> WKEPCRI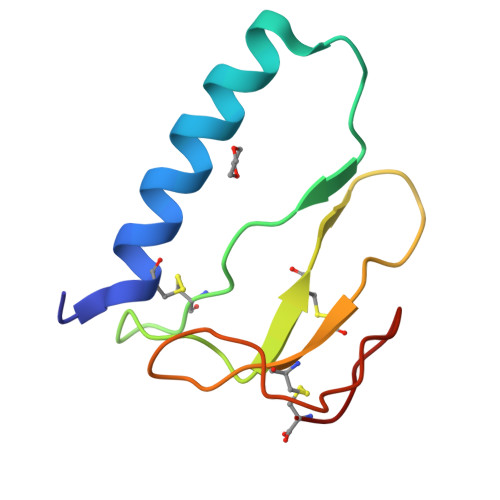ELYRVVESLAKAQETSGEEISKFYLPNCNKNGFYHSRQCETSMDGEAGLCWCVYPWNGKRIPGSPEIRGDPNC> MLPRETDEEPEEPGRRGSFVEMVDNLRGKSGQGYYVEMTVGSPPQTLNILVDTGSSNFAVGAAPHPFLHRYYQRQLSSTYRDLRKGVYVPYTQGKWEGELGTDLVSIPHGPNVTVRANIAAITESDKFFINGSNWEGILGLAYAEIARPDDSLEPFFDSLVKQTHVPNLFSLQLCGAGFPLNQSEVLASVGGSMIIGGIDHSLYTGSLWYTPIRREWYYEVIIVRVEINGQDLKMDCKEYNYDKSIVDSGTTNLRLPKKVFEAAVKSIKAASSTEKFPDGFWLGEQLVCWQAGTTPWNIFPVISLYLMGEVTNQSFRITILPQQYLRPVED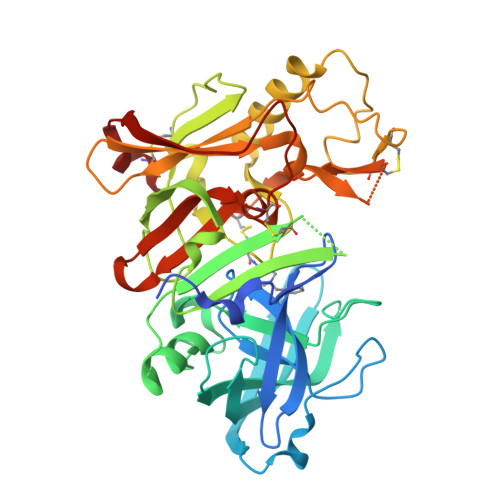VATSQDDCYKFAISQSSCGTVMGAVIMEGFYVVFDRARKRIGFAVSACHVHDEFRTAAVEGPFVTLDMEDCGYN> NDESILLLTFLGFTGLVAKYLAPAYKDFADARMKKVSDVLNASRNKHVEAVKDRIDSVSQLQNVAETTKVLFDVSKETVELESEAFE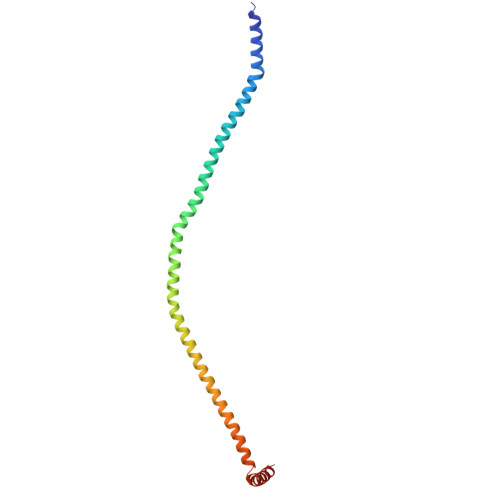LKQKVELAHEAKAVLDSWVRYEASLRQLEQRQLAKSVISRVQSELGNPKFQEKVLQQSISEIEQLLSK>[2x]MVSAPAFPTGLSAVLDSSGNTANLTWNAAPGANSYNVKRSTKSGGPYTTIATNIT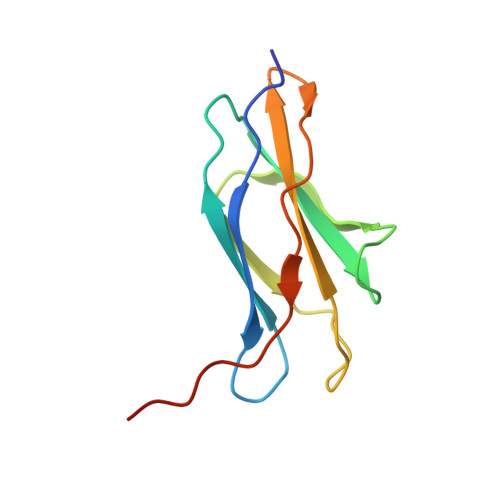STNYTDTGVATGTKYYYVVSAVSNGVETLNSAEAILQYPKLEHHHHHH>GSMSTINFANREINFKIVYYGPGLSGKTTNLKWIYSKVPEGRKGEMVSLATEDERTLFFDFLPLDIGEVKGFKTRFHLYTVPGQVFYNASRKLILRGVDGIVFVADSAPNRLRANAESMRNMRENLAEYGLTLDDVPIVIQVNKRDLPDALPVEMVRAVVDPEGKFPVLEA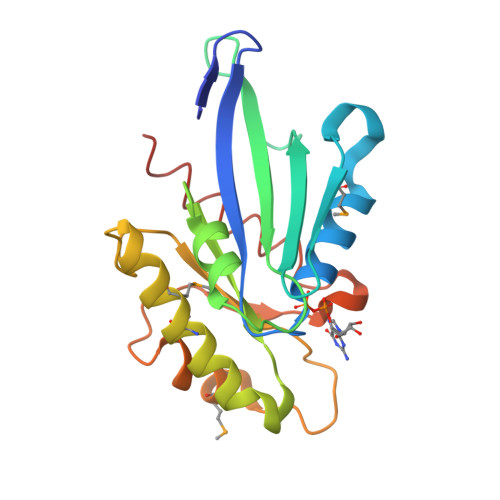VATEGKGVFETLKEVSRLVLARVAGGS[4x]> LTLGNTTSSVILTNYMDTQYYGEIGIGTPPQTFKVVFDTGSSNVWVPSSKCSRLYTACVYHKLFDASDSSSYKHNGTELTLRYSTGTVSGFLSQDIITVGGITVTQMFGEVTEMPALPFMLAEFDGVVGMGFIEQAIGRVTPIFDNIISQGVLKEDVFS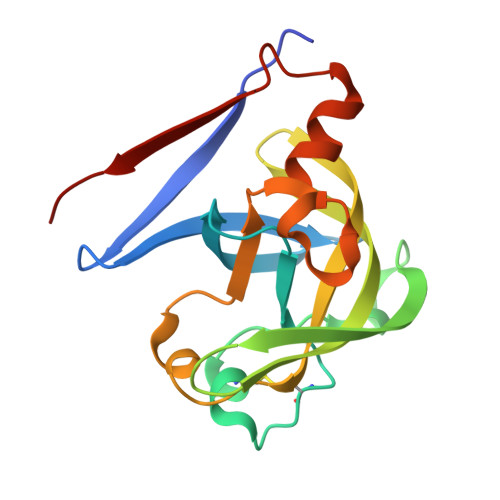FYYNRDS>[4x]MSQHNEKNPHQHQSPLHDSSEAKPGMDSLAPEDGSHRPAAEPTPPGAQPTAPGSLKAPDTRNEKLNSLEDVRKGSENYALTTNQGVRIADDQNSLRAGSRGPTLLEDFILREKITHFDHERIPERIVHARGSAAHGYFQPYKSLSDITKADFLSDPNKITPVFVRFSTVQGGAGSADTVRSIRGFATKFYTEEGIFDLVGNNTPIFFIQDAHKFPDFVHAVKPEPHWAIPQGQSAHDTFWDYVSLQPETLHNVMWAMSDRGIPRSYRTMEGFGIHTFRLINAEGKATFVRFHWKPLAGKASLVWDEAQKLTGRDPDFHRRELWEAIEAGDFPEYELGFQLIPEEDEFKFDFDLLDPTKLIPEELVPVQRVGKMVLNRNPDNFFAENEQAAFHPGHIVPGLDFTNDPLLQGRLFSYTDTQISRLGGPNFHEIPINRPTCPYHNFQRDGMH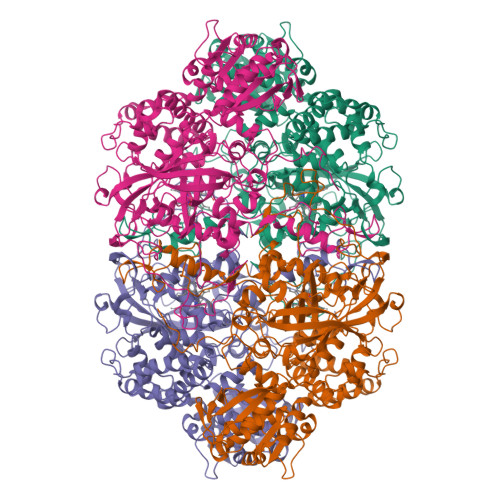RMGIDTNPANYEPNSINDNWPRETPPGPKRGGFESYQERVEGNKVRERSPSFGEYYSHPRLFWLSQTPFEQRHIVDGFSFELSKVVRPYIRERVVDQLAHIDLTLAQAVAKNLGIELTDDQLNITPPPDVNGLKKDPSLSLYAIPDGDVKGRVVAILLNDEVRSADLLAILKALKAKGVHAKLLYSRMGEVTADDGTVLPIAATFAGAPSLTVDAVIVPCGNIADIADNGDANYYLMEAYKHLKPIALAGDARKFKATIKIADQGEEGIVEADSADGSFMDELLTLMAAHRVWSRIPKIDKIPA1-TERT-BUTYL-3-(2,5-DIMETHYLBENZYL)-1H-PYRAZOLO[3,4-D]PYRIMIDIN-4-AMINE | C18 H23 N5 | 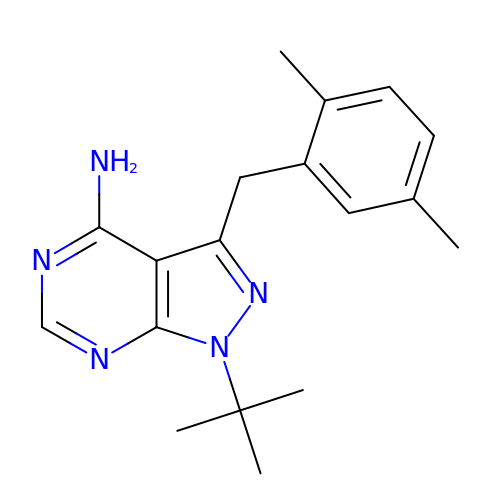QUPXEJURIFFVSX-UHFFFAOYSA-N> GSPHQPR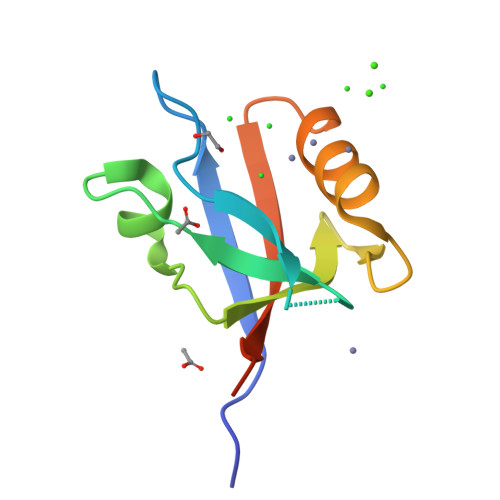VVVIKKGSNGYGFYLRAGPEQKGQIIKDIEPGSPAEAAGLKNNDLVVAVNGKSVEALDHDGVVEMIRKGGDQTTLLVLDKELERPHRD>QQTSGAGGATCSALPGSITLRSNAKLNDLFTMFNGDKVTTKDKFSCRQAEMSELIQRYELGTLPGRPSTLTASFSGNTLTINCGEAGKSISFTVTITYPSSGTAPYPAIIGYGGGSLPAPAGVAMINFNNDNIAAQVNTGSRGQGKFYDLYGSSHSAGAMTAWAWGVSRVIDALELVPGARIDTTKIGVTGCSRNGKGAMVAGAFEKRIVLTLPQESGAGGSACWRISDYLKSQGANIQTASEIIGEDPWFSTTFNSYVNQVPVLPFDHHSLAALIAPRGLFVIDNNIDWLGPQSCFGCMTAAHMAWQALGVSDHMGYSQIG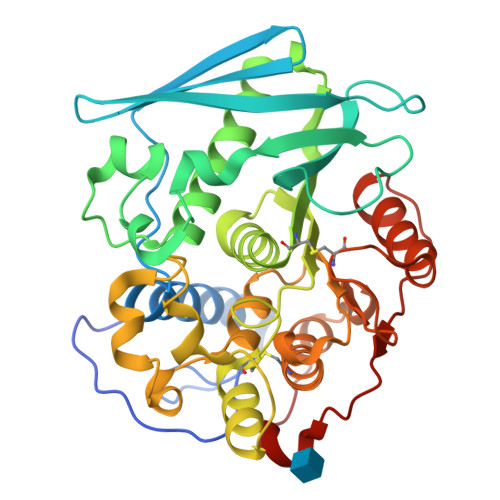AHAHCAFPSNQQSQLTAFVQKFLLGQSTNTAIFQSDFSANQSQWIDWTTPTLS[3x]> MRGSHHHHHHGSTMDIKPAFGTNQEDYASYIMNGIIKWGDPVTRVLDDGELLVQQTKNSDRTPLVSV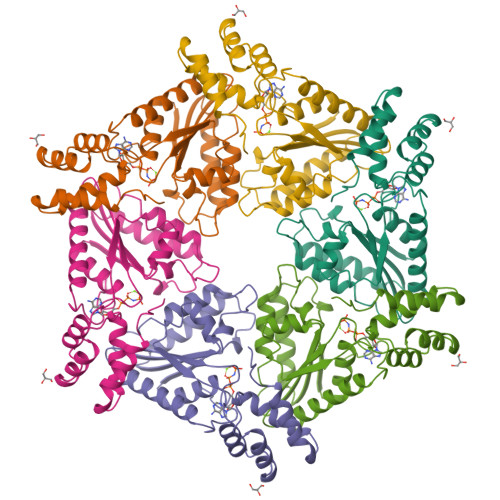LLEGPPHSGKTALAAKIAEESNFPFIKICSPDKMIGFSETAKCQAMKKIFDDAYKSQLSCVVVDDIERLLDYVPIGPRFSNLVLQALLVLLKKAPPQGRKLLIIGTTSRKDVLQEMEMLNAFSTTIHVPNIATGEQLLEALELLGNFKDKERTTIAQQVKGKKVWIGIKKLLMLIEMSLQMDPEYRVRKFLALLREEGASPLDFK> MKTSDANETEDHLESLICKVGEKSACSLESNLEGLAGVLEADLPNYKSKILRLLCTVARLLPEKLTIYTTLVGLLNARNYNFGGEFVEAMIRQLKESLKANNYNEAVYLVRFLSDLVNCHVIAAPSMVAMFENFVSVTQEEDVPQVRRDWYVYAFLSSLPWVGKELYEKKDAEMDRIFANTESYLKRRQKTHVPMLQVWTADKPHPQEEYLDCLWAQIQKLKKDRWQERHILRPYLAFDSILCEALQHNLPPFTPPPHTEDSVYPMPRVIFRMFDYTDDPEGPVMPGSHSVERFVIEENLHCIIKSHWKERKTCAAQLVSYPGKNKIPLNYHIVEVIFAELFQLPAPPHIDVMYTTLLIELCKLQPGSLPQVL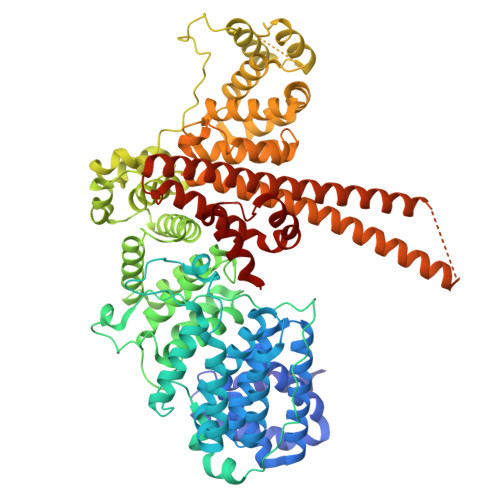AQATEMLYMRLDTMNTTCVDRFINWFSHHLSNFQFRWSWEDWSDCLSQDPESPKPKFVREVLEKCMRLSYHQRILDIVPPTFSALCPANPTCIYKYGDESSNSLPGHSVALCLAVAFKSKATNDEIFSILKDVPNPNQDDDDDEGFSFNPLKIEVFVQTLLHLAAKSFSHSFSALAKFHEVFKTLAESDEGKLHVLRVMFEVWRNHPQMIAVLVDKMIRTQIVDCAAVANWIFSSELSRDFTRLFVWEILHSTIRKMNKHVLKIQKELEEAKEKLARQHKRRSDDDDRSSDRKDGVLEEQIERLQEKVESAQSEQKNLFLVIFQRFIMILTEHLVRCETDGTSVLTPWYKNCIERLQQIFLQHHQIIQQYMVTLENLLFTAELDPHILAVFQQFCALQA> SNAMAKTLKDLQGWEIITTDEQGNIIDGGQKRLRRRGAKTEHYLKRSSDGIKLGRGDSVVMHNEAAGTYSVYMIQELRLNTLNNVVELWALTYLRWFEVNPLAHYRQFNPDANILNRPLNYYNKLFSETANKNELYLTAELAELQLFNFIRVANVMDGSKWEVLKGNVDPERDFTVRYICEPTGEKFVDINIEDVKAYIKKVEPREAQEYLKDLTLPSKKKEIKRGPQKKDKATQTAQISDAETRATDITDNEDGNEDESSDYESPSDIDVSEDMDSGEISADELEEEEDEEEDEDEEEKEARHTNSPRKRGRKIKLGKDDIDASVQPPPKKRGRKPKDPSKPRQMLLISSCRANNTPVIRKFTKKNVARAKKKYTPFSKRFKSIAAIPDLTSLPEFYGNSSELMASRFENKLKTTQKHQIVETIFSKVKKQLNSSYVKEEILKSANFQDYLPARENEFASIYLSAYSAIESDSATTIYVAGTPGVGKTLTVREVVKELLSSSAQREIPDFLYVEINGLKMVKPTDCYETLWNKVSGERLTWAASMESLEFYFKRVPKNKKKTIVVLLDELDAMVTKSQDIMYNFFNWTTYENAKLIVIAVANTMDLPERQLGNKITSRIGFTRIMFTGYTHEELKNIIDLRLKGLNDSFFYVDTKTGNAILIDAAGNDTTVKQTLPEDVRKVRLRMSADAIEIASRKVASVSGDARRALKVCKRAAEIAEKHYMAKHGYGYDGKTVIEDENEEQIYDDEDKDLIESNKAKDDNDDDDDNDGVQTVHITHVMKALNETLNSHVITFMTRLSFTAKLFIYALLNLMKKNGSQEQELGDIVDEIKLLIEVNGSNKFVMEIAKTLFQQGSDNISEQLRIISWDFVLNQLLDAGILFKQTMKNDRICCVKLNISVEEAKRAMNEDETLRNL;> MLNGEDFVEHNDILSSPAKSRNVTPKRVDPHGERQLRRIHSSKKNLLERISLVGNERKNTSPDPALKPKTPSKAPRKRGRPRKIQEELTDRIKKDEKDTISSKKKRKLDKDTSGNVNEESKTSNNKQVMEKTGIKEKREREKIQVATTTYEDNVTPQTDDNFVSNSPEPPEPATPSKKSLTTNHDFTSPLKQIIMNNLKEYKDSTSPGKLTLSRNFTPTPVPKNKKLYQTSETKSASSFLDTFEGYFDQRKIVRTNAKSRHTMSMAPDVTREEFSLVSNFFNENFQKRPRQKLFEIQKKMFPQYWFELTQGFSLLFYGVGSKRNFLEEFAIDYLSPKIAYSQLAYENELQQNKPVNSIPCLILNGYNPSCNYRDVFKEITDLLVPAELTRSETKYWGNHVILQIQKMIDFYKNQPLDIKLILVVHNLDGPSIRKNTFQTMLSFLSVIRQIAIVASTDHIYAPLLWDNMKAQNYNFVFHDISNFEPSTVESTFQDVMKMGKSDTSSGAEGAKYVLQSLTVNSKKMYKLLIETQMQNMGNLSANTGPKRGTQRTGVELKLFNHLCAADFIASNEIALRSMLREFIEHKMANITKNNSGMEIIWVPYTYAELEKLLKTVLNTL;> MSDLNQSKKMNVSEFADAQRSHYTVYPSLPQSNKNDKHIPFVKLLSGKESEVNVEKRWELYHQLHSHFHDQVDHIIDNIEADLKAEISDLLYSETTQKRRCFNTIFLLGSDSTTKIELKDESSRYNVLIELTPKESPNVRMMLRRSMYKLYSAADAEEHPTIKYEDINDEDGDFTEQNNDVSYDLSLVENFKRLFGKDLAMVFNFKDVDSINFNTLDNFIILLKSAFKYDHVKISLIFNINTNLSNIEKNLRQSTIRLLKRNYHKLDVSSNKGFKYGNQIFQSFLDTVDGKLNLSDRFVEFILSKMANNTNHNLQLLTKMLDYSLMSYFFQNAFSVFIDPVNVDFLNDDYLKILSRCPTFMFFVEGLIKQHAPADEILSLLTNKNRGLEEFFVEFLVRENPINGHAKFVARFLEEELNITNFNLIELYHNLLIGKLDSYLDRWSACKEYKDRLHFEPIDTIFQELFTLDNRSGLLTQSIFPSYKSNIEDNLLSWEQVLPSLDKENYDTLSGDLDKIMAPVLGQLFKLYREANMTINIYDFYIAFRETLPKEEILNFIRKDPSNTKLLELAETPDAFDKVALILFMQAIFAFENMGLIKFQSTKSYDLVEKCVWRGI;> SNAMTISEARLSPQVNLLPIKRHSNEEVEETAAILKKRTIDNEKCKDSDPGFGSLQRRLLQQLYGTLPTDEKIIFTYLQDCQQEIDRIIKQSIIQKESHSVILVGPRQSYKTYLLDYELSLLQQSYKEQFITIRLNGFIHSEQTAINGIATQLEQQLQKIHGSEEKIDDTSLETISSGSLTEVFEKILLLLDSTTKTRNEDSGEVDRESITKITVVFIFDEIDTFAGPVRQTLLYNLFDMVEHSRVPVCIFGCTTKLNILEYLEKRVKSRFSQRVIYMPQIQNLDDMVDAVRNLLTVRSEISPWVSQWNETLEKELSDPRSNLNRHIRMNFETFRSLPTLKNSIIPLVATSKNFGSLCTAIKSCSFLDIYNKNQLSNNLTGRLQSLSDLELAILISAARVALRAKDGSFNFNLAYAEYEKMIKAINSRIPTVAPTTNVGTGQSTFSIDNTIKLWLKKDVKNVWENLVQLDFFTEKSAVGLRDNATAAFYASNYQFQGTMIPFDLRSYQMQIILQELRRIIPKSNMYYSWTQL;> MNVTTPEVAFREYQTNCLASYISADPDITPSNLILQGYSGTGKTYTLKKYFNANPNLHAVWLEPVELVSWKPLLQAIARTVQYKLKTLYPNIPTTDYDPLQVEEPFLLVKTLHNIFVQYESLQEKTCLFLILDGFDSLQDLDAALFNKYIKLNELLPKDSKINIKFIYTMLETSFLQRYSTHCIPTVMFPRYNVDEVSTILVMSRCGELMEDSCLRKRIIEEQITDCTDDQFQNVAANFIHLIVQAFHSYTGNDIFALNDLIDFKWPKYVSRITKENIFEPLALYKSAIKLFLSTDDNLSENGQGESAITTNRDDLENSQTYDLSIISKYLLIASYICSYLEPRYDASIFSRKTRIIQGRAAYGRRKKKEVNPRYLQPSLFAIERLLAIFQAIFPIQGKAESGSLSALREESLMKANIEVFQNLSELHTLKLIATTMNKNIDYLSPKVRWKVNVPWEIIKEISESVHFNISDYFSDIHE;> MSMQQVQHCVAEVLRLDPQEKPDWSSGYLKKLTNATSILYNTSLNKVMLKQDEEVARCHICAYIASQKMNEKHMPDLCYYIDSIPLEPKKAKHLMNLFRQSLSNSSPMKQFAWTPSPKKNKRSPVKNGGRFTSSDPKELRNQLFGTPTKVRKSQNNDSFVIPELPPMQTNESPSITRRKLAFEEDEDEDEEEPGNDGLSLKSHSNKSITGTRNVDSDEYENHESDPTSEEEPLGVQESRSGRTKQNKAVGKPQSELKTAKALRKRGRIPNSLLVKKYCKMTTEEIIRLCNDFELPREVAYKIVDEYNINASRLVCPWQLVCGLVLNCTFIVFNERRRKDPRIDHFIVSKMCSLMLTSKVDDVIECVKLVKELIIGEKWFRDLQIRYDDFDGIRYDEIIFRKLGSMLQTTNILVTDDQYNIWKKRIEMDLALTEPL

The coordinated action of multiple replicative helicase loading factors is needed for the licensing of replication origins prior to DNA replication. Binding of the Origin Recognition Complex (ORC) to DNA initiates the ATP-dependent recruitment of Cdc6, Cdt1 and Mcm2-7 loading, but the structural details for timely ATPase site regulation and for how loading can be impeded by inhibitory signals, such as cyclin-dependent kinase phosphorylation, are unknown. Apart from Cdt1 and Orc6 (a subunit of ORC), all loading factors belong to the superfamily of ATPases Associated with various cellular Activities (AAA+). Here, we report cryo-EM structures of ARS1-bound S. cerevisiae (Sc) ORC and of the ternary complex with Cdc6 at sub-3 Å resolutions.

Our 2.55 Å resolution cryo-EM map of ScORC·DNA afforded the location of active-site water molecules (which were not resolved in any of the previous eukaryotic initiator structures due to lower resolutions) and a better definition of the side chain positions of active site residues. As expected, the conserved Walker A lysine of Orc1 (K485) bonds with the β- and γ-phosphate, while the Orc4 arginine finger (R267) and Orc1 sensor 2 arginine (R704) engage the γ-phosphate (and also the α-phosphate in case of the sensor 2). The Walker B aspartate (Orc1-D566) binds magnesium through two water molecules. The catalytic glutamate (Orc1-E567), a residue that activates a lytic water for nucleophilic attack of the γ-phosphate during catalysis, points towards the ATP γ-phosphate, its position stabilized by tether residues in Orc4, Y232, and R26332, and a bonding interaction with a water molecule in the magnesium coordination sphere. Surprisingly, the side chain of sensor 1 (Orc1-N600), a conserved polar residue in AAA+ ATPases that supports ATP hydrolysis by helping to activate the lytic water and/or by bonding with the ATP γ-phosphate, is flipped away from ATP. Apart from the magnesium-coordinating waters, two additional ordered water molecules are observed in the active site in a cavity near the γ-phosphate (W1 and W2). W1 hydrogen bonds with the catalytic glutamate, while both W1 and W2 also directly bond with the γ-phosphate. However, neither of the ordered waters is correctly positioned for an in-line attack on the γ-phosphate. Together, these findings argue that the Orc1·Orc4 ATPase in DNA-bound ScORC prefers to reside in a pre-hydrolysis conformation. Thus, we predict that the following rearrangements are needed for ATP hydrolysis: (1) a rotamer switch of the sensor 1 residue, (2) repositioning of at least one of the ordered water molecules in the active site for an in-line attack, and (3) a slight shift of the Orc4-R263 tether may also be needed.The second mRNA vaccine candidate (LS-P2-VP8*) encodes a multimerization domain derived from Aquifex aeolicus lumazine synthase (LS)35 fused to P2-VP8*. LS from this hyperthermophilic bacterium naturally self-assembles into 60-mer icosahedral nanoparticles. LS-based approaches have successfully been employed in other vaccine studies to display antigens on the nanoparticle surface, thereby significantly improving the immunogenicity of the presented antigens. The success of these studies is likely due to the fact that multimerization of antigens on a nanoparticle surface favors the generation of potent, long-lived immunoprotection in germinal centers through clustering of B cell receptors for multiple and simultaneous binding to the antigen epitopes.

In order to characterize LS-P2-VP8* P nanoparticles translated from mRNA in cell culture, supernatants of cells transfected with LS-P2-VP8* P were purified by density gradient ultracentrifugation and analyzed by transmission electron microscopy (TEM). mRNA encoding lumazine synthase alone (LS only) was employed as control. The pooled gradient fractions were analyzed using negative stain EM, which showed a uniform distribution of spherical particles with hollow interiors. A cryo-EM structure of LS-P2-VP8* P nanoparticles was determined at 2.6 Å resolution (at 0.143 F.S.C cutoff). In the 2D class averages generated from the LS-P2-VP8* P nanoparticle dataset, image classes were observed that show diffuse, nonuniform density protruding from nanoparticle surface, which may correspond to the P2-VP8* portion. However, ordered density corresponding to P2-VP8* was not visible in the cryo-EM map. Only a short segment of unoccupied density in the cryo-EM map at the end of the C-terminus of LS was observed where the P2-VP8* moiety is expected to be present. Since LS and P2-VP8* are fused via a flexible protein linker, it seems likely that the P2-VP8* protein portion cannot be clearly visualized on the surface of the LS nanoparticle structure due to this flexibility. The 60-mer LS-P2-VP8* nanoparticle core is ~15 nm in diameter with ~2 nm distance between adjacent VP8* protein as measured between the positions of C-terminal LS residue from the cryo-EM structure. Our data indicate that the protein translated from an mRNA encoding an LS nanoparticle domain fused to P2-VP8* P is secreted in vitro and self-assembles into 60-mer nanoparticles.

>MEIYEGKLTAEGLRFGIVASRFNHALVDRLVEGAIDCIVRHGGREEDITLVRVPGSWEIPVAAGELARKEDIDAVIAIGVLIRGATPHFDYIASEVSKGLANLSLELRKPITFGVITADTLEQAIERAGTKHGNKGWEAALSAIEMANLFKSLR[60x]> AL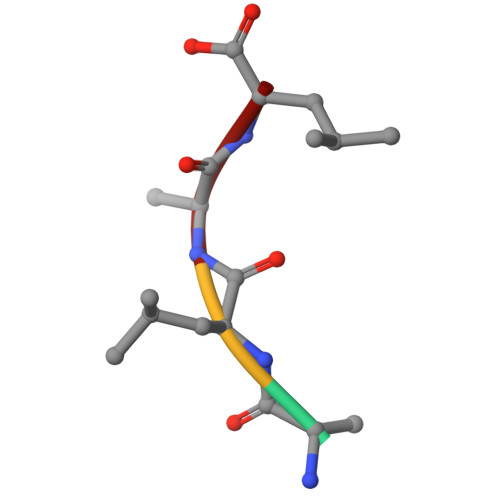AL Cefazolin | C14 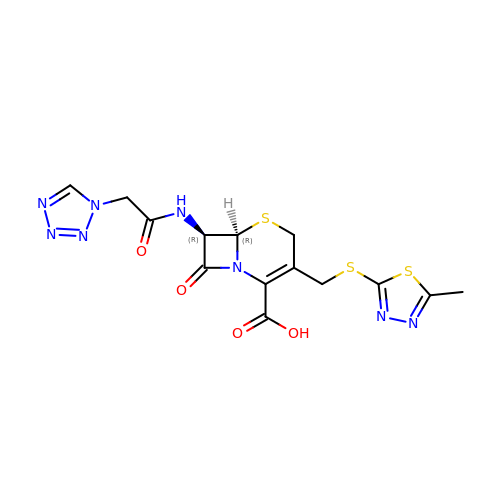H14 N8 O4 S3 | MLYYVTUWGNIJIB-BXKDBHETSA-N>[2x]MKHHHHHHHMVSTLKPLKIGKHTIKFPIFQGGMGVGISWDELAGNVAKEGALGVISAVGTGYYKNMRFVERIVAKKPFEALNFYSKKALNEIFANARKICGNNPLGANILYAINDYGRVLRDSCEAGANIIITGAGLPTNMPEFAKDFSDVALIPIISSAKALKILCKRWSDRYKRIPDAFIVEGPLSGGHQGFKYEDCFKEEFRLENLVPKVVEASKEWGNIPIIAAGGIWDRKDIDTMLSLGASGVQMATRFLGTKECDAKVYADLLPTLKKEDILLIKSPVGYPARAINTGVIKRIEEGNAPKIACVSNCVAPCNRGEEAKKVGYCIADGLGRSYLGNREEGLYFTGANGYRVDKIISVHELIKELTEG;>GTSSMGYLMALFEDIQAVIAEQLNVDAAQVTPEAEFVKDLGADSLDVVELIMALEEKFGIEIPDEQAEKIVNVGDVVKYIEDNKLA[2x]

The bifunctional dehydrogenase/isomerase FabX is an essential UFA biosynthesis enzyme in the widespread human pathogen Helicobacter pylori, a bacterium etiologically related to 95% of gastric cancers. FabX belongs to the nitronate monooxygenase (NMO) flavoprotein family but contains an atypical [4Fe-4S] cluster absent in all other family members characterized to date. We demonstrate that the [4Fe–4S] cluster functions as a temporary electron depot that receives electrons from FMN and sends electrons back to FMN to achieve independent bidirectional internal electron transfer.

We obtained crystal structures of FabX–holo-ACP complex at 2.8 Å resolution with space group P21 and FabX–octanoyl-ACP complex at 2.3 Å resolution with space group P212121. In the FabX–octanoyl-ACP structure, one of the complexes in the asymmetric unit is well determined, while the ACP in the other complex only shows the key α2 helix. Octanoyl-ACP binds FabX predominantly via electrostatic and hydrophobic interactions between its highly conserved α2-helix and the α7-helix of FabX. M44′ and E47′ of the C-terminus of ACP α2-helix induce significant sidechain rotations of R160 and R164 located on the FabX α7-helix C-terminus through forming salt-bridge interactions between E47′ and R160. Moreover, D56′ from the α3-helix of ACP forms additional salt-bridges with R164 of FabX. In contrast, in the FabX–octanoyl-ACP complex, the sidechain of D56′ of ACP α3-helix inserts into the chink between helices α6 and α7 of FabX. This pushes away the sidechain of N131 located on the loop between α6 and β4, and forms additional hydrophilic interactions with FabX R164 and T130. The anticlockwise rotation of ACP on the α7-helix of FabX poises the octanoyl chain plus the thioester proximal portion of the PPant prosthetic group to insert into the “L” shaped hydrophobic tunnel of FabX through the oxyanion hole between FMN and H182. In the FabX–octanoyl-ACP complex, the PPant is stabilized predominantly through hydrophobic interactions with the FabX sidechains of S149, I147, Y277 plus the backbones of G127 and G184. In addition to the PPant–FabX interactions, the octanoyl chain attached to PPant is stabilized in the tunnel through hydrophobic interactions with surrounding residues including G25, V26, V49, G50, F74, Y75, L101, H182, V305, I321, L325, and F339.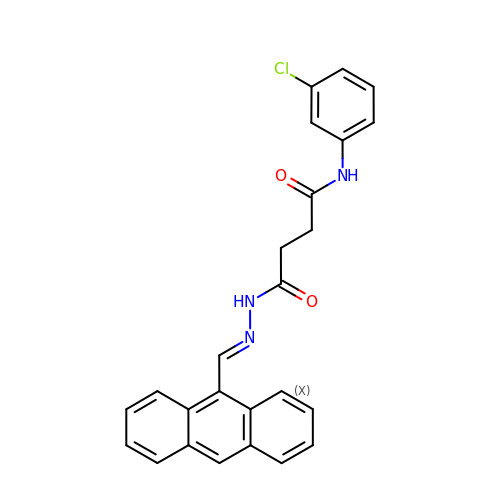4-[2-(anthracen-9-ylmethylidene)hydrazino]-N-(3-chlorophenyl)-4-oxobutanamide | C25 H20 Cl N3 O2 | OJLFRDWWYAPUAJ-JVWAILMASA-N The SLC39A protein family contains 14 members (SLC39A1 through SLC39A14) that transport zinc ions from the extracellular space and organelles into the cytoplasm, while the SLC30A protein family contains ten members (SLC30A1 through SLC30A10) that transport zinc ions from the cytoplasm into the organelles and the extracellular space. The mammalian SLC30A1 gene was cloned in 1995 and subsequently found to be expressed ubiquitously in the plasma membrane. Interestingly, we found that SLC30A1 is localized to the basolateral membrane of the intestine, where it controls zinc efflux from enterocytes into the circulation. Finally, an integrative analysis of the cryo‐EM structure and site‐specific mutagenesis of human SLC30A1 are performed and a zinc transport mechanism of SLC30A1 unique within the SLC30A family, with His43 serving as a critical residue for zinc selectivity, is identified.

Therefore, we expressed and purified the full‐length human SLC30A1 protein and then resolved the structure at 3.7‐Å resolution using cryo‐EM. The resulting structure indicates that SLC30A1 forms a homodimer, with each subunit consisting of a TMD with six transmembrane helices (TM1‐TM6), an extracellular domain (ECD), and an intracellular C‐terminal domain (CTD). The overall structure shows that the SLC30A1 homodimer is relatively compact, with the TM helices in each subunit forming symmetrical helical bundles and TM2, TM3, and TM6 contributing to the formation of the dimer interface. Under basal conditions, we found that each protomer in the SLC30A1 dimer contains four putative zinc‐binding sites (Z1 through Z4) located in the TMD and CTD. The Z1 and Z2 zinc‐binding sites are located in the TMD, possibly forming the zinc transport pathway; in contrast, Z3 and Z4 are located in the CTD, where they likely sense intracellular free zinc ions and form the starting point for zinc transport. Among the four zinc‐binding sites, Z2 is the most conserved, with a zinc ion connecting TM2 and TM5 via four coordinated residues (His43, Asp47, His251, and Asp255). Moreover, a zinc ion in Z3 stabilizes the CTD‐CTD interaction via His408 and His413 in one protomer and Cys437 in the other protomer. Finally, the Z4 site resides in a highly negatively charged cavity comprised of His370, His387, Glu420, and Cys433. We also found that Cys291 in the helical domain in the ECD of each protomer forms a disulfide bond, which stabilizes the dimer conformation and is essential for SLC30A1 function. We, therefore, propose a model for the zinc transport pathway for SLC30A1 based on electrostatic potential and zinc‐binding sites; this model of zinc efflux reflects a novel dimer‐dependent mode of zinc transport that may be unique to SLC30A1 and has not been reported previously for any other cation diffusion facilitators.

>[2x]MGCWGRNRGRLLCMLALTFMFMVLEVVVSRVTSSLAMLSDSFHMLSDVLALVVALVAERFARRTHATQKNTFGWIRAEVMGALVNAIFLTGLCFAILLEAIERFIEPHEMQQPLVVLGVGVAGLLVNVLGLCLFHHHSGFSQDSGHGHSHGGHGHGHGLPKGPRVKSTRPGSSDINVAPGEQGPDQEETNTLVANTSNSNGLKLDPADPENPRSGDTVEVQVNGNLVREPDHMELEEDRAGQLNMRGVFLHVLGDALGSVIVVVNALVFYFSWKGCSEGDFCVNPCFPDPCKAFVEIINSTHASVYEAGPCWVLYLDPTLCVVMVCILLYTTYPLLKESALILLQTVPKQIDIRNLIKELRNVEGVEEVHELHVWQLAGSRIIATAHIKCEDPTSYMEVAKTIKDVFHNHGIHATTIQPEFASVGSKSSVVPCELACRTQCALKQCCGTLPQAPSGKDAEKTPAVSISCLELSNNLEKKPRRTKAENIPAVVIEIKNMPNKQPESSL> GVTGATPKAKKAAQSSAQLEGSYIFCMNPLLDKLSDEDIREQLKAFVTGKTDSIRTDTELSFDIYVSETDYALIRYADSLCERLNDAGADVQIK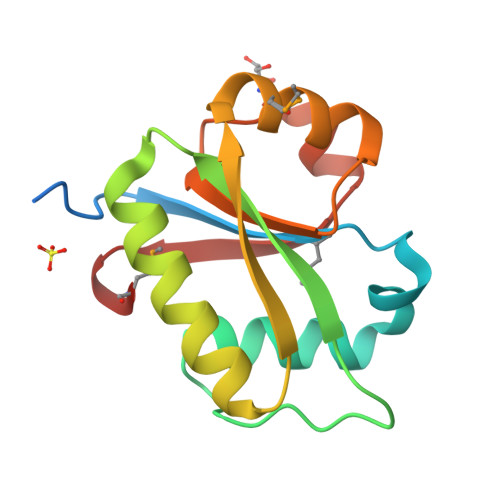QYSGTMLRSRAVSGKYEAFLSESDLVSTDALENADYIILDSAEMR> MNALVGCTTSFDPG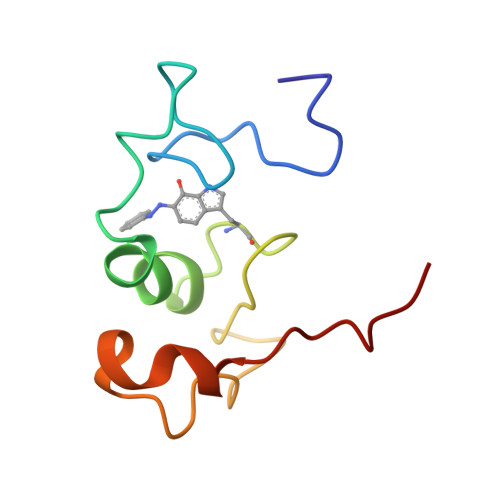WEVDAFGAVSNLCQPMEADLYGCADPCWWPAQVADTLNTYPNWSAGADDVMQDWRKLQSVFPETK6-(thiophen-3-yl)quinolin-2-amine | C13 H10 N2 S | 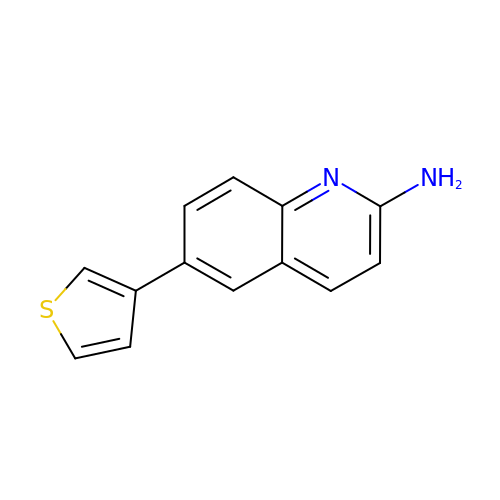SKHMHSCEONTQTF-UHFFFAOYSA-N> SSGSGHMARILAFDIGISSIGWAFSENDELKDCGVRIFTKVENPKTGESLALPRRLARSARKRLARRKARLNHLKHLIANEFKLNYEDYQSFDESLAKAYKGSLISPYELRFRALNELLSKQDFARVILHIAKRRGYDDIKNSDDKEKGAILKAIKQNEEKLANYQSVGEYLYKEYFQKFKENSKEFTNVRNKKESYERCIAQSFLKDELKLIFKKQREFGFSFSKKFEEEVLSVAFYKRALKDFSHL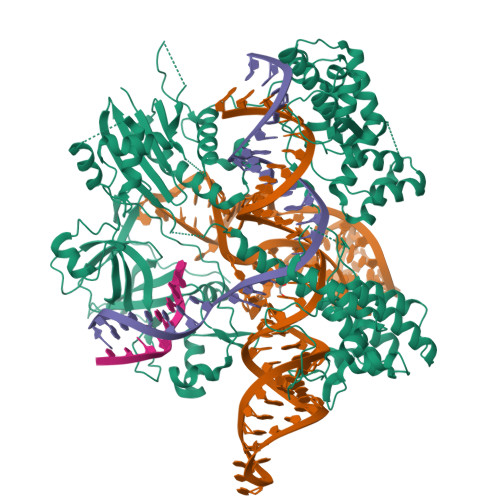VGNCSFFTDEKRAPKNSPLAFMFVALTRIINLLNNLKNTEGILYTKDDLNALLNEVLKNGTLTYKQTKKLLGLSDDYEFKGEKGTYFIEFKKYKEFIKALGEHNLSQDDLNEIAKDITLIKDEIKLKKALAKYDLNQNQIDSLSKLEFKDHLNISFKALKLVTPLMLEGKKYDEACNELNLKVAINEDKKDFLPAFNETYYKDEVTNPVVLRAIKEYRKVLNALLKKYGKVHKINIELGGGSGGYIARLVLNYTKDYLDFLPLSDDENTKLNDTQKGSKVHVEAKSGMLTSALRHTWGFSAKDRNNHLHHAIDAVIIAYANNSIVKAFSDFKKEQESNSAELYAKKISELDYKNKRKFFEPFSGFRQKVLDKIDEIFVSKPERKKPSGALHEETFRKEEEFYQSYGGKEGVLKALELGKIRKVNGKIVKNGDMFRVDIFKHKKTNKFYAVPIYTMDFALKVLPNKAVARSKKGEIKDWILMDENYEFCFSLYKDSLILIQTKDMQEPEFVYYNAFTSSTVSLIVSKHDNKFETLSKNQKILFKNANEKEVIAKSIGIQNLKVFEKYIVSALGEVTKAEFRQREDFKK> MPDNEVDLLFAQLSPEDLIEWSDYLPESFTDRALAQMGERQRQRFELYDQYSENEIGRYTDHQMLVLSDKATVAQAQRFFRRIELDCNDNLFIVDEADKYLGTVRRYDIFKHEPHEPLISLLSEDSRALTANTTLLDAAEAIEHSREIELPVIDD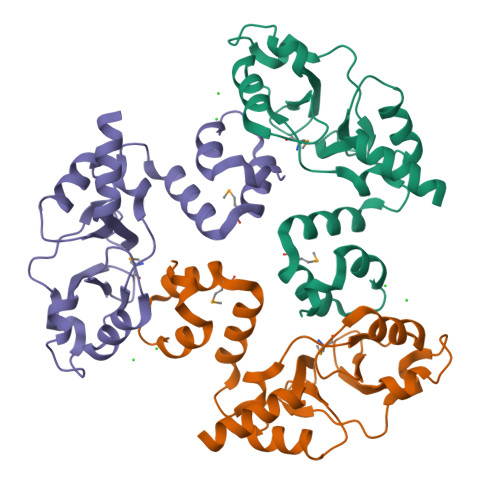AGELIGRVTLRAATALVREHYEAQLMATAGMDESDDLFAPILKGAQRRAV> MMTGQVPILVLKEGTQREQGKNAQRNNIEAAKAIADAVRTTLGPKGMDKMLVDSIGDIIISNDGATILKEMDVEHPTAKMIVEVSKAQDTAVGDGTTTAVVLSGELLKQAETLLDQGVHPTVISNGYRLAVNEARKIIDEIAEKSTDDATLRKIALTALSGKNTGLSNDFLADLVVKAVNAVAEVRDGKTIVDTANIKVDKKNGGSVNDTQFISGIVIDKEKVHSKMPDVVKNAKIALIDSALEIKKTEIEAKVQISDPSKIQDFLNQETNTFKQMVEKIKKSGANVVLCQKGIDDVAQHYLAKEGIYAVRRVKKSDMEKLAKATGAKIVTDLDDLTPSVLGEAETVEERKIGDDRMTFVMGCKNPKAVSILIRGGTDHVVSEVERALNDAIRVVAITKEDGKFLWGGGAVEAELAMRLAKYANSVGGREQLAIEAFAKALEIIPRTLAENAGIDPINTLIKLKADDEKGRISVGVDLDNNGVGDMKAKGVVDPLRVKTHALESAVEVATMILRIDDVIASKKSTPPSGQGGQ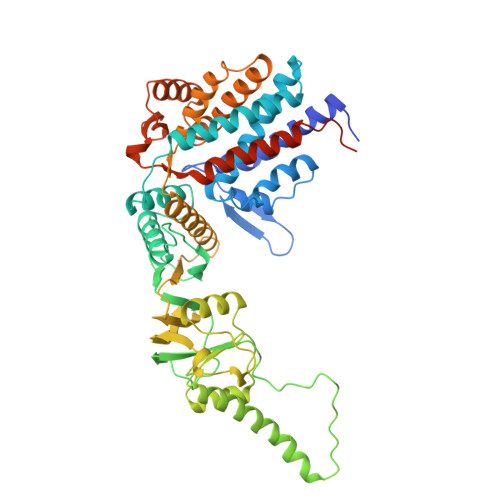GQGMPGGGMPEY> MSSKSQDSDDWQYEECKLSRTGPPAT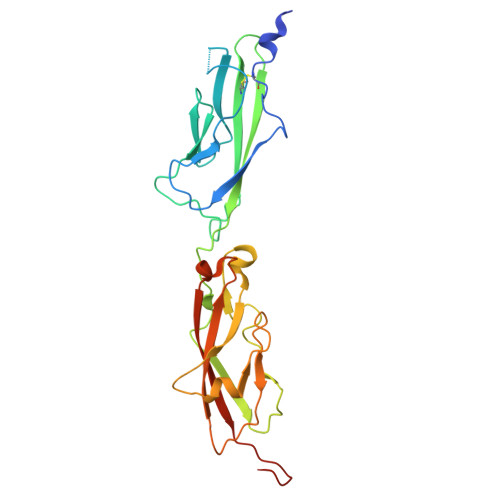IVAIDEESPNGTVLVENMQINGRAEDPHRTISLSLRDNYGHWVILDPVKQRLYLNSTGRVLDRDPPSYIHSIVVQVQCTNELVGTVILHEVRIVVRDRNDNPPRFQQPRYYVAINELTPVGTTIFSGFSGNNGAVDIDDGPNGQIEYTIQYNPYDPTANRTFDIPLTLSGSVVLRERLNYEEITRYLVIIQANDRAPDPKERLTATTTLTVDVLDGDDLGPLEHHHHHH> GSHMIKSSFKAQPFLVRNTILCPNDKRSFTEYTQVIETVSKNKVFLEQLLLANPKLYDVMQKYNAGLLKKKRVKKLFESIYKYYKRSYLRSTPFGLFSETSIGVFSKSSQYKLMGKTTKGIRLDTQWLIRLVHKMEVDFSKKLSFTRNNANYKFGDRVFQVYTINSSELEECNIKYTNVYQIISEFCENDYQKYEDICETVTLCYGDEYRELSEQYLGSLIVNHYLISNLQKDLLSDFSWNTFLTKVEAIDEDKKYIIPLKKVQKFIQEYSEIEIGEGIEKLKEIYQEMSQILENDNYIQIDLISDSEINFDVKQKQQLEHLAEFLGNTTKSVRRTYLDDYKDKFIEKYGVDQEVQITELFDSTFGIGAPYNYNHPRNDFYESEPSTLYYSEEEREKYLSMYVEAVKNHNVINLDDLESHYQKMDLEKKSELQGLELFLNLAKEYEKDIFILGDIVGNNNLGGASGRFSALS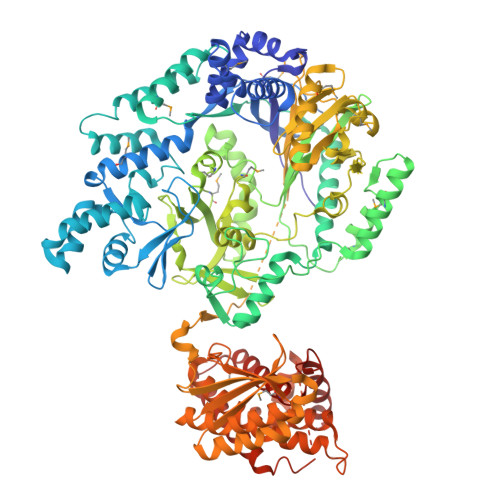PELTSYHRTIVDSVERENENKEITSCEIVFLPENIRHANVMHTSIMRRKVLPFFTSTSHNEVLLTNIYIGIDEKEKFYARDISTQEVLKFYITSMYNKTLFSNELRFLYEISLDDKFGNLPWELIYRDFDYIPRLVFDEIVISPAKWKIWGRDVNSKMTIRELIQSKEIPKEFYIVNGDNKVYLSQKNPLDMEILESAIKKSSKRKDFIELQEYFEDENIINKGEKGRVADVVVPFIRTRALGNEGRAFIREKRVSVERREKLPFNEWLYLKLYISINRQNEFLLSYLPDIQKIVANLGGNLFFLRYTDPKPHIRLRIKCSDLFLAYGSILEILKRSRKNRIMSTFDISIYDQEVERYGGFDTLELSEAIFCADSKIIPNLLTLIKDTNNDWKVDDVSILVNYLYLKCFFQNDNKKILNFLNLVSTKKVKENVNEKIEHYLKLLKVNNLGDQIFYDKNFKELKHAIKNLFLKMIAQDFELQKVYSIIDSIIHVHNNRLIGIERDKEKLIYYTLQRLFVSEEYMK> MTENILRKSDEEIQKEITARVKALESMLIEQGILTTSMIDRMAEIYENEVGPHLGAKVVVKAWTDPEFKKRLLADGTEACKELGIGGLQGEDMMWVENTDEVHHVVVCTLCSCYPWPVLGLPPNWFKEPQYRSRVVREPRQLLKEEFGFEVPPSKEIKVWDSSSEMRFVVLPQRPAGTDGWSEEELATLVTRESMIGVEPAKAVA;> MNGVYDVGGTDGLGPINRPADEPVFRAEWEKVAFAMFPATFRAGFMGLDEFRFG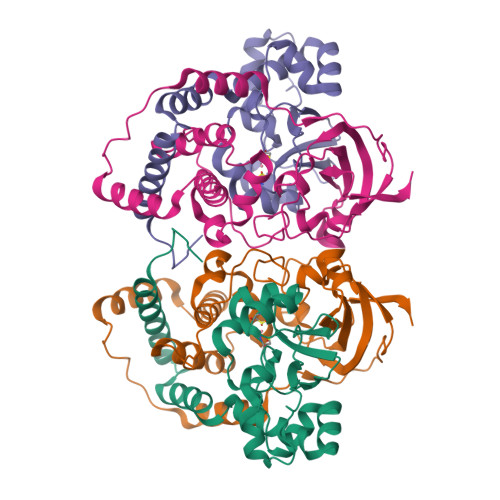IEQMNPAEYLESPYYWHWIRTYIHHGVRTGKIDLEELERRTQYYRENPDAPLPEHEQKPELIEFVNQAVYGGLPRSREVDRPPKFKEGDVVRFSTASPKGHARRARYVRGKTGTVVKHHGAYIYPDTAGNGLGECPEHLYTVRFTAQELWGPEGDPNSSVYYDCWEPYIELVDTKAAAA>SKSTAEIRQAFLDFFHSKGHQVVASSSLVPHNDPTLLFTNAGMNQFKDVFLGLDKRNYSRATTSQRCVRAGGKHNDLENVGYTARHHTFFEMLGNFSFGDYFKLDAILFAWLLLTSEKWFALPKERLWVTVYESDDEAYEIWEKEVGIPRERIIRIGDNKGAPYASDNFWQMGDTGPCGPCTEIFYDHGDHIWGGPPGSPEEDGDRYIEIWNIVFMQFNRQADGTMEPLPKPSVDTAMGLERIAAVLQHVNSNYDIDLFRTLIQAVAKVTGATDLSNKSLRVIADHIRSCAFLIADGVMPSNENRGYVLRRIIRRAVRHGNMLGAKETFFYKLVGPLIDVMGSAGEDLKRQQAQVEQVLKTEEEQFARTLERGLALLDEELAKLSGDTLDGETAFRLYDTYGFPVDLTADVCRERNIKVDEAGFEAAMEEQRRRAREASGF[4x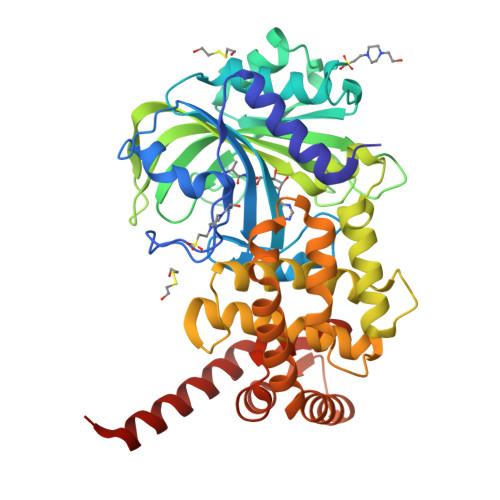]>[2x]GSFVGSIDQGTTSSRFLIFNGEGNPVASHQIEFENLYPKSGWHEQDPYELLNSVQQCIDGAMHKFASLGYSKENIRAIGITNQRETTVVWDSVTGEPLHNAIVWPDTRTSALVRELKARQSADSLLELCGLPLSTYPSSVKLLWLIQNVDAVKQAYEEGRLAFGTVDSWL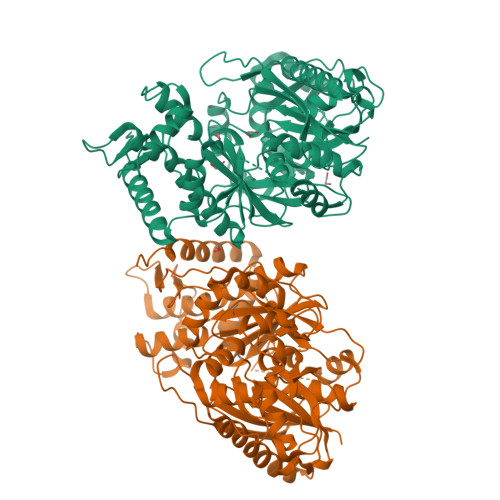IYKLNGGAQAERPIHVTDSTNASRTMFMNLRTLQYDDKLLGFFGIDRNKIKLPKIVPSSDPEAFGKVATGALAGVPIAGCLGDQSSALVGQCGFSPGQAKNTYGTGCFLLYNVGTEPVISKYGLLATVAYDFGRGRKPVYALEGSIAVAGAGITFLMNNLGFAPKPSEINALAESVLDNGGVVFVTAFSGLFAPYWIDDAKGTLFGITQHTTKGHIARATLEATCYQTRAILDAMEKDSGHKLESLAVDGGLSASDLCMQTQADISGIPVDRPRMRETTALGAAIAAGLATGVWRELDHVKESIAGGANGNGKKNAREVFYPKMDRKKAERLFRKWEQAVEMSRGWVREQEEEDGE1-(4-fluoranylspiro[2~{H}-indole-3,1'-cyclobutane]-1-yl)ethanone | C13 H14 F N O | 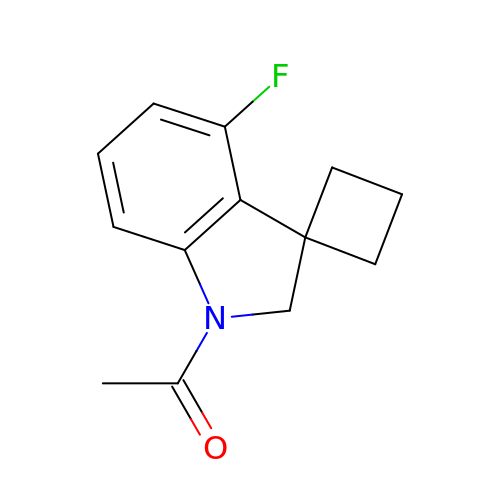WXJBYBVEXXHQQN-UHFFFAOYSA-N> MNSRLFRFDVVRTHFGDHGLESSTIGCPADTLYSALCVEALRMGGQQLLDELVACSTLRLTDLLPYVGPDYLVPKPLKSVRSDSSSLQKKLAKKIGFLPAAQLGSFLDGTADLDDLAARQTKIGVHAVSAKAAIHNGKKDADPYRVGYFRFEPDAGLWLLATGSESELGLLTRLLKGISALGGERTSGFGAFIPTESEVPAALTPTTAAASLMTLTTSLPTDDELEQALAGATYRLVKRSGFVASATYAETPRRKRDIYKLAAGSVFSRPFQGGILDVS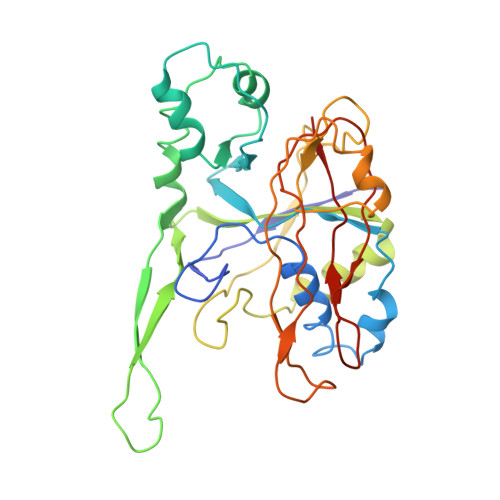LGGNHPVYSYARPLFLALPESAA> MQKRTLYNAMTPAQRYFVEGEHVVQAEANRDILFTQLDSNSYLPVLHYVLVGTALGVVFLVLPLLIAPARVDLDKISAYECGFDAFGEARETFSVSFYIVSIMYLLFDIEVVYLIPYVMTNATEYMYWVMQTFVAILVGGFFYEWRMGALEWRE;> MNLNIIMTVLPLLVSVAFLTLSERAVMGSLQRRMGPAVSGAFGILQPFWDGFKLAVKEPILPANAAAGIFYAAPLICICICVASWCTLLLTDLSIGGLFLLLLSSLAVYGVLLAGYSCNSKYAFLGCLRSVSLMISYELVISVVILCVILETRDGNGFPCLNLTETASQTKIILIPAGLLFYICSL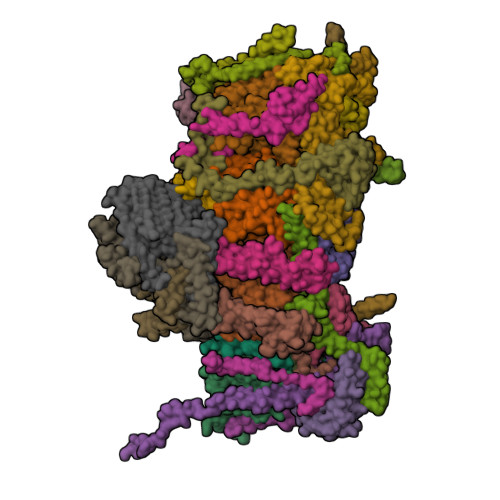AESKRVPFDLPEAEAELVAGYNVEYSSLGFAVFFVAEYGNTLLMAALINIYFLGKLNSALIAAIFVSFIWVRGTLPRYRYDMFMQIGWKSLLPVALALYLAQASLGY;> MLLIYIMLSNIVVLALSVVLTSSPFMALMYSILLYLNVQTILWSLGYDFMALIYALVYVGALAVLFLFVVMMVRIQVSTLSTKTIQSVLSWLAIILIFSYGDVSFSFPCGAESLLNFGTQLYSSCSDLTLLNSLALTIALFGSLV;> MLSSVVAPQQPLSIAQPFAVRGYHNDAEFLGAVYNFSIRSVFITGILGAVYWRRNLITMLLCSEIAFIACSVNFLYASAYLNDMAGMLFSITITTISACETALGLALCVGYFQSRAANEVEALNLLK;> MFLLAVYFLFFSAIANGFFGRYLGVRGSQLLGPSALFLALLCSGTIFYEVCIQGCSTNIKLFENFVYSNELNVSASFLYDPLAATMTLTVVWISCAVHAYQNLYMRGDGSQTLFTSYLSAFTGFMLILVAGQNLVMLFIGWEGIGVCSYLLIGYYGSRVSAVKSANKSLIVNKISDGFLLGSMLYLWFYTGSFSYCSLATFQIPDVVSILVLLGAIGKSSQLFFHVWLADAMEGPTPVSALIHAATLVTAGIYVLCKLNLHSQSAVGILGAATALMGGLFGLAANDLKRVIAFSTCSQLGYMMAVLSTCDDGADFAMGHLVSHAGFKATLFLSAGLSIAKENNNFLNRYGSRQGSPTLSFATTIASLNLLGFPELGGFYSKESILNNAYINQGVSIILTLATFLTAFYTSKVLAQLYLFPYGNGRQQKSFDIDATTLICFGLLLSEMLLRIFTGSSLSQNMTTNLPAHIKNLPFWVALSGALSGLATTNLFSSNFMRFFGNRGGFDVFYARKCSNVFYHNAYVSYTLLDRGFLKLY;> MSLYLFMLFLQPLSLSFVSRSFSKISSLMMSFATLWSAVYMWFTSNGANQTFYQVVSWGSDWSTFGVCYTSLYISLLCAFIFPICVILVQGYRALSILICIQTAVSLSIVSLHMLAFYALFESSLLLFFILIGRRKYGSLSAAYNISIYTFISALGFLISAFWLNWSFGSVCALLPNEEANSFVAFGIFILLWVKAPLVPFHLWLPEAHVYAPTAGSVLLAGVLLKISIVGLHVFFLPICASSIVKAFPLILSICLGSFIFSSFSTLKQIDLKKIVAYSSISHMAIVFLSSATNSGLGIQGAVLYCIAHGLISPGLFLLVGILYKNTNTKLVFYLRGLSQQAPVWWSVWVFFMLGNLAFPLFPNFIAEVVCLSALFKNHELYAYAFIFFSFVGTVYSSTVLGRLKGGVSSQCVDASRLDVISWNPLVLATVVTGIGYM;> MWENLWYLDILINVLIITIFGLISCSSSATKSYDLKGCFIISMVGGVYDIPSAILWCLASLSILNFNGFFASLFLVFTWISNLFAMQSLNFLGIYLAFEMQSLCLLVLGKITANENQRWFAYRGLLKYLVLSLIAGSIFIFHASSSYLQSGVMISDSLVTYVFLLFKLGVAPFHMYTLELFSVVSRHVAFVFSTLPKLSVLYLISNSNIGSECVWWGLISLWLGSISQYQSVFVRSILLYSSVAEIGLVLLVLQEGFSWEAFSWVSIYFLSLSGVWHANSKFVSAISVASIAGLPPFLGFIGKAQILKSLVSINLGILIFSSILAATISFIGYLRLIRLMYLVSPVKWKNNKDSSFINWSTWMLTVGTLPMVYSV;> MALLRALAKPLRSLQAVSSVAQVSLRQFGAASHHDDHHDDHDHYTPPKTVFEDTITINVLDYDGKKHAVKALIGTPLNKALVEYGFSSTYFFPNMGYYTQHISDAHVFIPEEYWKYVENVDLKTDDAEAIKLMFKLVVQDYQRETSFFASYLTLNKEMDNMTIGFGPIKPWHITPKWSFNGHHNVKDRMFDRLETGPFIE;> MALSSASSFFKAVVLRNLRVSVSQSTFVPIGNVISRAYGGHGLDRDTVTERVIHVAKHFEKVDPNKITPTATFEELGLDSLDTVELVMALEEEFGLEIPDNEADKITTMADAISYVVSNPLAK;> MVARVPYSHELYAMAKHIVFRNEKEHNAILECKAQHDWPEDCKPESEAIVRATNKLFQDIMQKAPEEFKDYAKCLDWYGLKFSKCREKQAAFEAAFPLSE;> MTFNYVIPYGGSSSYTINNEPVKAEEVTVDFSKEPSASSLKLADKSDWIAYTFNNVPLMATVGLLAGAHEAFLHYERTPIYGKRTYNIIKKLAPIVINKTAYATLLGAIFCATDALYENYSGKKSYTSGMVAGAATGAVFAIGRPLPQPLVWPLVFAAAPVIADLFGEVYPESMKSARGYGTPYGFENLDDAVPTRNPIRRNPHHY;> MTEFVNRGFPGLKSIKDLPKVQDVPPPGGFPSIRIERKLPNTGPTGLAVFLGFTAFMALAVNQARDRKSTNRLEAEEVYTARSILHPILQAEWDLRYLEHQRKEREDEAKIMKDVPGWKVGEATSRRRWLPPVESFDVRPLI;> MGWYALPSYVIVSAAWAAGFWAIDTYQIYKEGKPSWNQNKDQFQRALYRRDWYLRREQETIGMFLGFDYGA;> MGGHDHHHPSVPEPPYAKYLANKSHYCPPDFHYSREIYAPYGGYFNDPKGWRTNTAIATLVMLAGAYAVFCFGNAREERLRAPKGWIPSQLWNDNVPTPVDYRGKVLKDE;> MGWEYAGTYGALCGMVYAIGSNVISGRAWFRRPWVHVTSVTLSYLGSKLLDEVQDTYYLEHLKRVERKGLQVTEEHKKLFSAY;> MSGFGLQSGTARCYDWYMDYLKCMDESKAPMITLRKQECSEWLEDYNECLHRDKLKLRKLLIEREKNKQEAASSS;> MTWPKPINPYDVPSSPAYHRLQEPSYPVIDKDPDFWTAVSNVRKEEWGTTAAVAAGTFVMGYYLGAKGHTGKASAYFTSFLATKSITLYHAYNSADRLMGFKENSREVVKNVPAALVPEHY;> MNRIPALRRIGAQALRNPVTRAGGASGHPNGSFWSEGTQVGLNGFKYGEIPLPNGQPRKKLWLENIWNIGYGGFFLGAFCLYYGAPPGHVIPSQWATPKAKDEYAVDMKMIDKYNERPDLQARLSIVLKDLNMIEEEAYDLIMMRKDYKVLLGLHSGRVPADLKAIYEELEA;> MAGGNYASLKADTSMDHVFGDSTNKLNYDFQLMSSKEAFFWNYTLYPIVGFPIFLYLYQFNKLENFEAEIAAAKAAKAASE;> MFFFEFLQGKISDSQKEVDSQAEWYAEYDKLEKARQKRRIWKWRDSDSRDEYAINAEEPVIYIRSSLFGRTEVDPTGKNTNRNHQYLYNLKVLGHKTYTRRDPNELQKAQAEVDTLSAAGRLGPLSPF;> MSSKIGFQWEKYEAWRYHPLLRFNKNTMFPGVGLGAAAFAVYYVVDTLSGDKSHH;> MSLTLGLRSLSRGALAARNALPKRAGAGGPVKLSPPVDKPLPYNYDFWMDNGIYPGQPIYDGMFGSMVGNMSLEYMAKGWLVLLPILSAPFVYEHCIADDVTRNPFVPRQYPSEVREFLALFKNGFVLNDYSQPDYEEMKRRQSGLLTPIY;> MSALQAVKNLTTRMRPFAFQQIRKASNSSRIAGDTTGKYTPNIFSPETPMDRSFSHVPKNPFWEAWVFRRDNIQREFVWTWQTIFDLATFVGGLYVAMYATASFCSRQNDKRNGYPERNYYFSDSKSNFVIPDEREFY;> MASEAVLRLPHKLRVMRMYRTGLKEIVNWSYGRHEFYPRANALRMEFEANKELSDREQIRKLVLHGEDLLARFRHWEPTIRSEFVGGTVYGVWPQHCKDVKFVPNPAYIDEFKQGDTVLLY;> MADRFPPPKMVATQEEMDNADIPYKYRDYCAHLIIDFKECRYGHPLTWRINCAHELHHYNKCSYIEFKRRVAIAIEEKKRRGLMV;> MTTATIEERRAFHKEVLDIVQSKLANKNSEWARPEEPILHNLKSEKEEPHVYYHNNNFRVTRQLIHFEKTKIFEDELDKCMRTHGEAKYRKCQEIAKRFQASCRVASNLERGPNARKRDVGFIYQNNKLRELEKDAKELGLNNPFPPSSPRTTIGY;> MVKTLADYIHWRNKPSSIPPVDEYRPPVPLVNYDKLSTQFFSKLDNDPVINRVLRAPKVTVMATSLPIVNHPAFLFVAGALTGFSLTYAITSHYVGRKEIENLVKFDPRYFPEYTKSS;> MRSALRLANATRLSTFRLTSAPAVRLASPSFFVQKEDEENTRSIHTSNSSFHDEPKHQIPGNALDNWAFLRTYAKPLPDMIHYYYYVYLFGFFFVYKVADFPEYSPRVLVMAALIGSLFYVRRDWVHREFKDSP;> MLRRGAKELVQLLRTPVKQGAQLQYVATRNVNFYDAPNGPAVEQVKIEDEWYNRQRTEFNILNKQPSKADDVFIAPNAVVCGDVDLYQKVSIFFGAVVRGDLNTIRIGENSTILDKAVVHAASTSPTGLNAATIIGSNVTVEPHAVLRSCRIGDNCIVGARSVVCEGAIMHPESVLAPGSVLAPGRQIPSGELWAGSPAKFVRKLTYYETSNVIRESAEHYYDIATGFRNETFDHGSAWRDAEAYRQKLVDYKEYNWVNYREQKYVMRLQRDAAELEKLL;> MSLLKNYPPSYLYPFRHPKPEGVIEKVLFNLGSLFRSAGQGMDELGSLMLGNGGMQESVGPNLAYAPVKYNPAAAPKAGIVAPIPASAQRVLGVKEIVLPSKAESTFIAPNANVLGDVKIGAKSSIWYGAVLRGDVNSIEIGDNTNVQDNVTIHVAKHSIDGKLRNTVIGNNVTIGHCATIHACTIADNVIIGMGATVLDGVKVESGSIVGAGSIVPPNTVIPAGQVWVGNPAKFIRNVLPEENGFIASSANNYDLLGQQHKFENSKVFEEMLVEEEIAKDRELLEDKNLAVHQLYIFDPQTQLAARPRR;> MASFLKTIVWRCGFAIKETGLALETLGCKLQGNYSFREKCSRHTPLTQYQFKAPSVGESTFVAPSALVSGDVIIGEKSSVLYNAVVRGEFKSVTIGEGSTISDNAYVGSSSEFSPETVIGSNVSVGSGAVLKGCTVGNNVLIGNNVIISEKATVEDNTILAPGSYVPEDVVVKSGELWSGSPAQKLRNLDEKELALFNTLSVGATELAADHAVIMKLLELKQKEFIK> GTSEKEQQEAIEHIDEVQNEIDRLNEQASEEILKVEQKYNKLRQPFFQKRS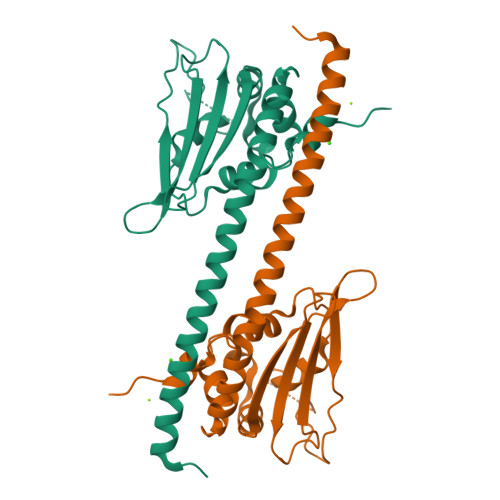ELIAKIPNFWVTTFVNHPQVSALLGEEDEEALHYLTRVEVTEFEDIKSGYRIDFYFDENPYFENKVLSKEFHLNESGDPSSKSTEIKWKSGKDLTKRSSQTQNKASRKRQHEEPESFFTWFTDHSDAGADELGEVIKDDIWPNPLQYYLVPDM> GMSAPV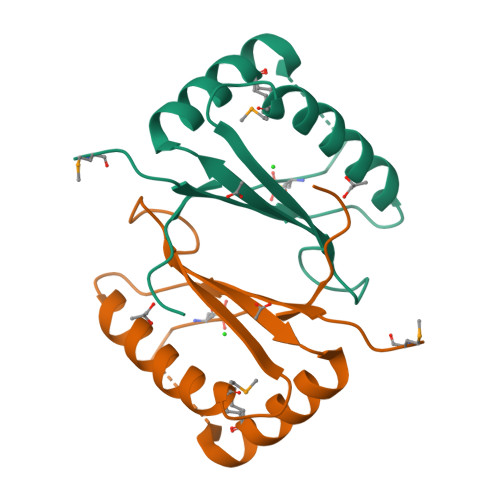TLINPFKVPADKLEAAIEYWEAHRDFMAQQPGYLSTQLHQSIDEGATYQLINVAIWQSEADFYQAAQKMRQALGHVQVEGLCGNPALYRVIRT Cdp-DG(16:0/16:0) | C44 H81 N3 O15 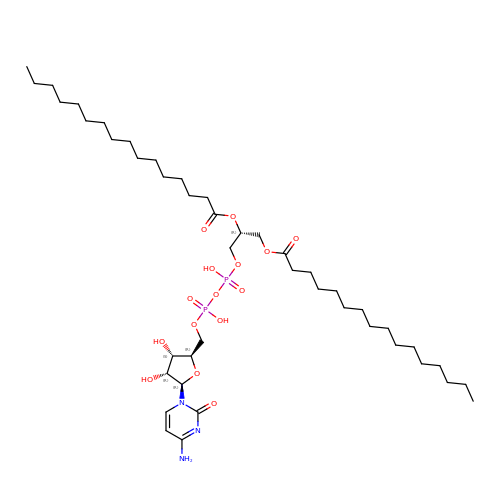P2 | ITYHVANGBZMQML-BQUKFSKHSA-N(5~{R},6~{R})-6-[(~{E})-5-[(2~{S},3~{S},5~{R})-5-(2-hydroxyethyl)-3,5-dimethyl-oxolan-2-yl]-3-methyl-2-oxidanylidene-pent-3-enyl]-5-propyl-oxane-2,4-dione 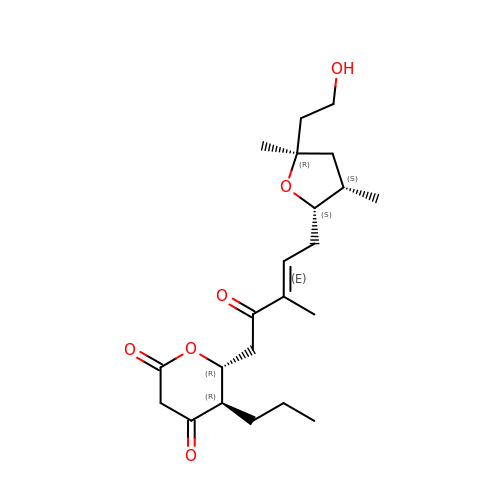| C22 H34 O6 | MVJVJKSGEMISOL-HXEGTYTISA-N Here, we show that Pseudomonas aeruginosa OprC is an outer membrane, TonB-dependent transporter that is conserved in many Proteobacteria and which mediates acquisition of both reduced and oxidised ionic copper via an unprecedented CxxxM-HxM metal binding site. As indicated by the successful structure solution, OprC contains a single bound copper and shows the typical fold of a TBDT, with a large 22-stranded β-barrel occluded by an N-terminal approximately 15 kDa plug domain that, like in other TBDTs, completely occludes the lumen of the barrel. The copper binding site comprises residues Cys143 and Met147 in the plug domain and His323 and Met325 in the barrel wall. The CxxxM-HxM configuration, which coordinates the copper in a tetrahedral manner, is highly unusual and has, to our knowledge, not been observed before in copper homeostasis proteins.

We next asked whether OprC also binds Cu(I). Since it is challenging to maintain copper in its +1 state during crystallisation, we used silver (Ag(I)) as a proxy for Cu(I) and determined the co-crystal structure of WT OprC in the presence of 2 mM AgNO3. This is possible because the protein used for crystallisation only had approximately 60% copper occupancy. Data were collected at 8,000 eV, at which energy the anomalous signal of copper is very small (0.6 e−, compared to 4.2 e− for Ag). Strikingly, and in sharp contrast to Cu(II), the anomalous map of OprC WT crystallised in the presence of silver shows not one but 3 anomalous peaks. The first, very strong peak (Ag1; 23σ) is located at the same site as in OprC crystallised with Cu(II) and is coordinated by the same residues (Cys143, Met147, His323, and Met325). The other 2 silver sites have lower occupancies (Ag2, approximately 10σ and Ag3, approximately 10σ) and are each coordinated by 3 methionines of the methionine track (Met286, Met339, and Met343 for Ag2; Met341, Met343, and Met348 for Ag3), as seen also, for example, for Cu(I) in the Ctr1 copper transporter. Only 5 Met residues form the 2 sites (Met343 is shared between the two), and this, combined with the fact that the track has 11 or 12 methionines, suggests that there are more than 2 metal binding sites. The distance between Ag2 and Ag3 is approximately 6.5 Å, i.e., large enough for 2 metal ions to be bound simultaneously, consistent with the fact that Ag was present at approximately 10-fold excess during crystallisation (approximately 0.2 mM OprC and 2 mM Ag). While direct measurement of the affinities of the methionine binding track sites would be challenging, the structural data suggest that the methionine track provides at least 2, and possibly more, binding sites for Ag(I), and, by extension, for Cu(I).

>[2x]MEKRMSTQQRAAGNACPTAAFSFDPARLAQRRRWAGAFAALCGLALSPSALLAEEHSQHQDHAVELAPSVVTGVAQSSPLTIVTNPKEPRQPVPASDGADYLKTIPGFAVIRNGGSNGDPVLRGMFGSRLNILTNGGMMLGACPNRMDAPTSYISPETYDKLTVIKGPQTVLWGPGASAGTILFEREPERFGELGSRVNASLLAGSNGRFDKVLDAAAGNRLGYLRFTGNHAQSDDYEDGAGNTVPSRWKKWNGDVAVGWTPDEDTLIELTAGKGDGEARYAGRGMDGSQFKRESLGLRFVKSNVSDVLEKVEAQVYYNYADHIMDNFRLRTPDPSSMMPMPMASQVDRRTLGGRLAATWRWDDFKLVTGVDAMRNEHRARGSKYDMMTDYYTDADQFPWSKDAVFHNYGAFGELTWFAAERDRLIGGLRLDRASVKDYRQTLKSGHMGHAMANPTANDTRADTLPSGFVRYEHDLADSPTTLYAGLGHAERFPDYWELFSPKRGPNGSVNAFDKIKPEKTTQLDFGLQYNGDKLQAWASGYVGVVQDFILFSYREGMMGSSTQATNVDARIMGGELGASYQLTGNWKTDASLAYAWGKNSSDDRALPQIPPLEARFGLTYEEGDWSAGSLWRVVAPQNRIARDQGNVVGKDFDKSAGFGVFSLNGAYRVTRNVKLSAGVDNLFDKDYTEHLNKAGDAGFGFSANETVPEPGRTFWTKVDFSF> MPDLGTPIGSVTDSSPSLIRIEISSAEDFEKYKSMLGVGQYLLVASGNNLYLLASITGVRATHVERRSLGPSSEVHSEEGSDGISGNFRFQIDTQPIGTLSEDGEFSRGSHSLPVPTEYAYVTPPAVLEGIFSHQIKSPFALGTLGISPDIKLKIDGDRFFSKHVAVVGSTGSGKSCAVAKILQTAVGIESKANAHKAAQKNSHIVIFDIHAEYAAAFNLEAGEAFTLNLLGVDNLRLPYWLMNAQELEQIFIESNEHNSHNQISQFRHAVVRNKCKHNPTLTNLSFDTPVYFSIDEVVTYLENMNNEVIGKLAGEGKPKLANETLVSDRDELYFDAVQSFIVASQAAATKASNGPFNGEFDRMILRLHTRLADPRLQFLFYPKKEDGEDLATGDFADVVRQFVGYMTKSNVSIIDLSGIPFEVLSIVVSLISRMIFDFGFHYSKNRHVGGAVSDVPILVVCEEAHNYLPRSGGAAYDASRKSIERIAKEGRKYGVTLMVVSQRPSEVSETIFSQCSNFISLRLTNAVDQTYVKSL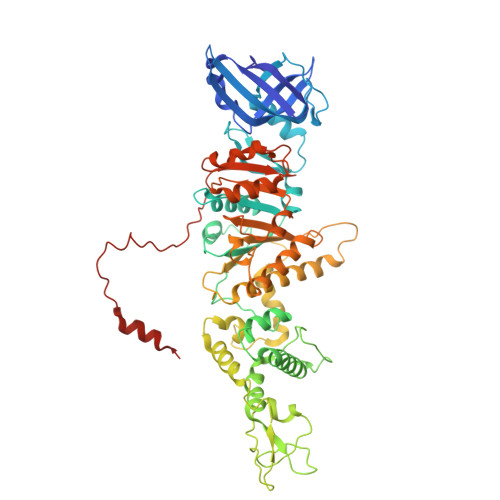LPDLSAGLGDLLPNLAQGEFLIVGDAPLMPTVGHFALPVPEPHSRSVNYLQEWNSGWRHVDFDSVIDRWRGKVLTKSEKGV> MPEQYRYTLPVKAGEQRLLGELTGAACATLVAEIAERHAGPVVLIAPDMQNALRLHDEISQFTDQMVMNLADWETLPYDSFSPHQDIISSRLSTLYQLPTMQRGVLIVPVNTLMQRVCPHSFLHGHALVMKKGQRLSRDALRTQLDSAGYRHVDQVMEHGEYATRGALLDLFPMGSELPYRLDFFDDEIDSLRVFDVDSQRTLEEVEAINLLPAHEFPTDKAAIELFRSQWRDTFEVKRDPEHIYQQVSKGTLPAGIEYWQPLFFSEPLPPLFSYFPANTLLVNTGDLETSAERFQADTLARFENRGVDPMRPLLPPQSLWLRVDELFSELKNWPRVQLKTEHLPTKAANANLGFQKLPDLAVQAQQKAPLDALRKFLETFDGPVVFSVESEGRREALGELLARIKIAPQRIMRLDEASDRGRYLMIGAAEHGFVDTVRNLALICESDLLGERVARRRQDSRRTINPDTLIRNLAELHIGQPVVHLEHGVGRYAGMTTLEAGGITGEYLMLTYANDAKLYVPVSSLHLISRYAGGAEENAPLHKLGGDAWSRARQKAAEKVRDVAAELLDIYAQRAAKEGFAFKHDREQYQLFCDSFPFETTPDQAQAINAVLSDMCQPLAMDRLVCGDVGFGKTEVAMRAAFLAVDNHKQVAVLVPTTLLAQQHYDNFRDRFANWPVRIEMISRFRSAKEQTQILAEVAEGKIDILIGTHKLLQSDVKFKDLGLLIVDEEHRFGVRHKERIKAMRANVDILTLTATPIPRTLNMAMSGMRDLSIIATPPARRLAVKTFVREYDSMVVREAILREILRGGQVYYLYNDVENIQKAAERLAELVPEARIAIGHGQMRERELERVMNDFHHQRFNVLVCTTIIETGIDIPTANTIIIERADHFGLAQLHQLRGRVGRSHHQAYAWLLTPHPKAMTTDAQKRLEAIASLEDLGAGFALATHDLEIRGAGELLGEEQSGSMETIGFSLYMELLENAVDALKAGREPSLEDLTSQQTEVELRMPSLLPDDFIPDVNTRLSFYKRIASAKTENELEEIKVELIDRFGLLPDPARTLLDIARLRQQAQKLGIRKLEGNEKGGVIEFAEKNHVNPAWLIGLLQKQPQHYRLDGPTRLKFIQDLSERKTRIEWVRQFMRELEENAIA

The transcription-repair coupling factor (TRCF) recognizes paused/stalled RNAPs and either rescues transcription or initiates transcription termination. The bacterial TRCF – Mfd is a multi-domain adaptor protein consisting of seven domains connected by flexible linkers. Domains 5 and 6 together form the motor domain, representing a (helicase) superfamily II ATPase that exhibits structural homology to the RecG translocase. Further, biophysical studies revealed that the motor domain of Mfd binds and partially melts DNA containing a template strand overhang.

To further understand how Mfd binds template strand overhang–containing DNA, we visualized Mfd bound to the dye-labeled smFRET substrate by cryo-EM. Full-length Mfd bound to the 5′ tailed substrate in the presence of transition-state analog ADP-AlFx was subjected to single particle cryo-EM analysis and a ∼5.2 Å resolution map was obtained (real resolution ∼8 Å). This reconstruction yielded EM density that could at best accommodate the motor domains of Mfd (residues 575–956 representing domains 5 and 6); other domains are presumably flexible and could not be seen in the EM density maps. In addition the reconstruction could accommodate 18 bp of dsDNA and 11 nt of the 5′ dT (template strand) overhang. The cryo-EM map reconstructed here suggests the dsDNA on the upstream side of the motor domains and the placement of the motor domains with respect to dsDNA to be consistent with previously reported complexes. However, EM density for residues 917 onward, containing the TRG motif, appeared to be absent from the side of domains 5 and 6, and the EM density of the DNA as it passes from the upstream to the downstream side becomes inconsistent with dsDNA. Using molecular dynamics flexible fitting to equilibrate the structure in density suggests that the TRG motif has dropped into the path of the dsDNA (yellow ribbon), resulting in the partial melting of the duplex with only 13 residues remaining double stranded. The motif forms an arch that interacts with the template DNA. The conformation of domains 5 and 6 suggested here may represent a mode of engagement whereby Mfd grabs and stabilizes the template DNA in the upstream edge of the transcription bubble, supporting the inferences drawn from the biophysical investigations. Additionally, the model suggests that Mfd partially melts about five nucleotides of the dsDNA near the junction forming a ‘TRCF bubble’.> MSIQHFRVALIPFFAAFCLPVFAHPETLVKVKDAEDQLGARVGYIELDLNSGKILESFRPEERFPMMSTFKVLLCGAVLSRIDAGQEQLGRRIHYSQNDLVEYSPVTEKHLTDGMTVRELCSAAITMSDNTAANLLLTTIGGP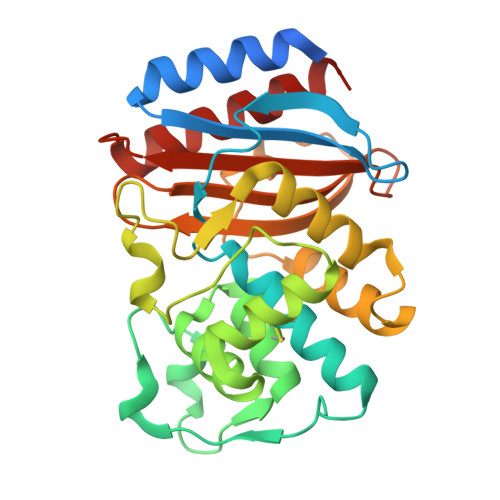KELTAFLHNMGDHVTRLDRWEPELNEAIPNDERDTTMPVAMATTLRKLLTGELLTLASRQQLIDWMEADKVAGPLLRSALPAGWFIADKSGAGERGSRGIIAALGPDGKPSRIVVIYTTGSQATMDERNRQIAEIGASLIKHW(S)-2-AMINO-5-(2-OXOACETIMIDAMIDO)PENTANOIC ACID | C7 H13 N3 O3 | 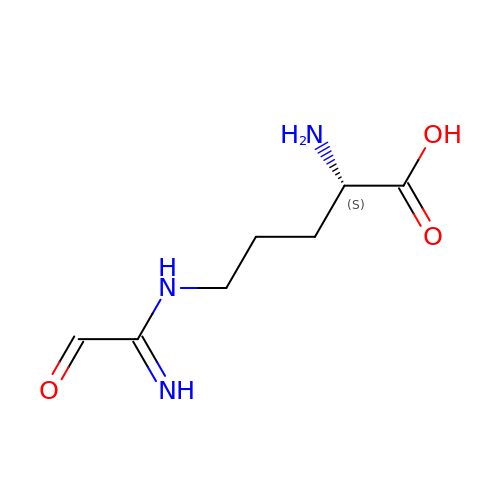JPSGSOHVMKIFBG-YFKPBYRVSA-N[(2~{R})-2-[2-(methylamino)ethoxy-oxidanyl-phosphoryl]oxy-2-(13-methyltetradecanoyloxy)ethyl] 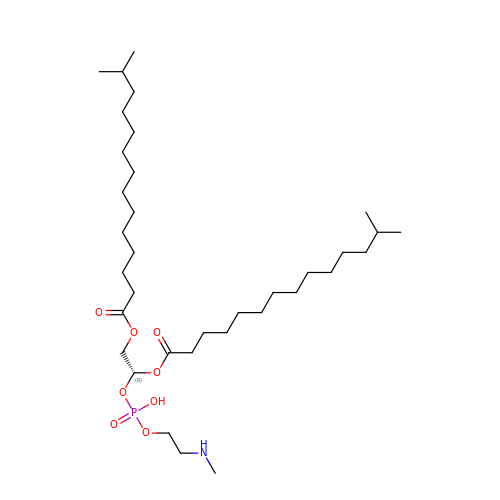13-methyltetradecanoate | C35 H70 N O8 P | JRBIDHJPLMRMHE-PGUFJCEWSA-N> MDLSTKQKQHLKGLAHPLKPVVLLGS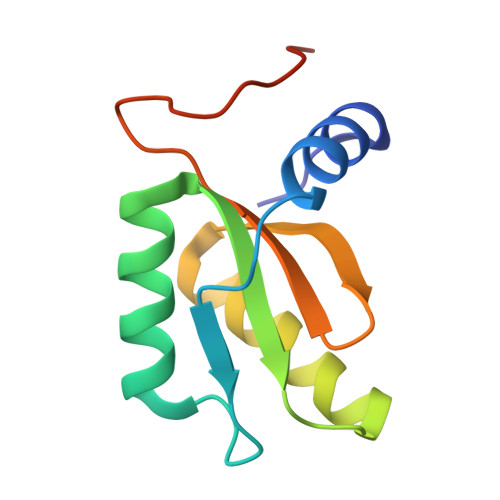NGLTEGVLAEIEQALEHHELIKVKIATEDRETKTLIVEAIVRETGACNVQVIGKTLVLYRPTKERKISLPLEHHHHHH> YQQDQIVKEDSVEAVGAQLKV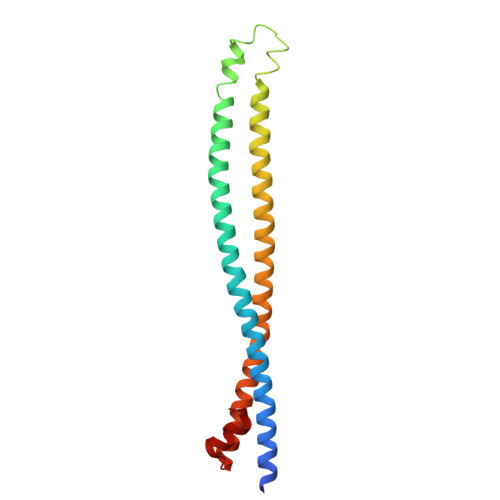YHQQYQDKSREYDQLYEEYTRTSQELQMKRTAIEAFNETIKIFEEQGQTQEKSSKEYLERFRREGNEKEMQRILLNSERLKSRIAEIHESRTKLEQELRAQASDNREIDKRMNSLKPDLMQLRKIRDQYLVWLTQKGARQKKINEWLGI~{N}-[(2~{S})-1-[(3~{R},3~{a}~{R},6~{R},6~{a}~{R})-6-ethynyl-3-oxidanyl-2,3,3~{a},5,6,6~{a}-hexahydrofuro[3,2-b]pyrrol-4-yl]-4-methyl-1-oxidanylidene-pentan-2-yl]-4-[5-fluoranyl-2-(4-methylpiperazin-1-yl)-1,3-thiazol-4-yl]benzamide 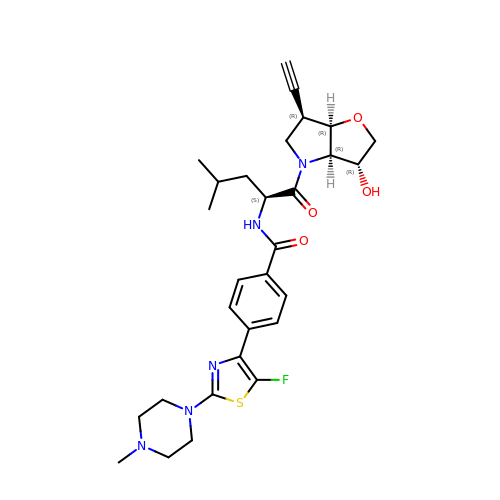| C29 H36 F N5 O4 S | LXQZJMLAONLFAB-KFGZMKLQSA-N>[4x]MDPFASTRTFNLAMTDIGEMYFMPPLMEALAQRAPHIQISTLRPNAGNLKEDMESGAVDLALGLLP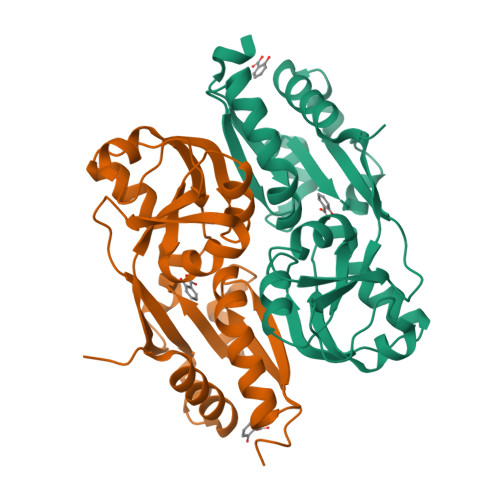ELQTGFFQRRLFRHRYVCMFRKDHPSAKSPMSLKQFTELEHVGVVALNTGHGEVDGLLERAGIKRRMRLVVPHFIAIGPILHSTDLIATVPQRFAVRCEVPFGLTTSPHPAKLPDIAINLFWHAKYNRDPGNMWLRQLFVELFSEAHHHHHH3-(3,4-dichlorophenyl)-1,1-dimethyl-urea | C9 H10 Cl2 N2 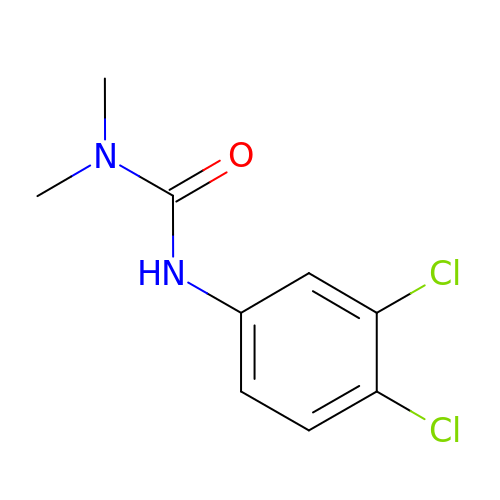O | XMTQQYYKAHVGBJ-UHFFFAOYSA-N> CELDRDPEGKDFQQPYTSFVQTKQNRDGLYALLRNTENPRMHFYQELQSDMYCTTITDGNSLAPFVNWDLGILNDHGRADEDEVSGIAGYYFVYNRLNQQANAFVNNTEAALQNQVYKNSTEIANAKSFLAEGKVLQALAIWRLMDRFSFHESVTEVNSGAKDLGVILLKEYNPGYIGPRATKAQCYDYILSRLSEAIEVLPENRESVLYVSRDYAYALRARIYLALGEYGKAAADAKMVVDKYPLIGAADASEFENIYRSDANNPEIIFRGFASATLGSFTATTLNGAAPAGKDIKYNPSAVPFQWVVDLYENEDFRKSVYIAKVVKKDKGYLVNKFLEDKAYRDVQDKPNLKVGARYFSVAEVYLILVESALQTGDTPTAEKYLKALSKARGAEVSVVNMEALQAERTRELIGEGSRLRDMVRWSIPNNHDAFETQPGLEGFANTTPLKAQAPVGFYAYTWEFPQRDRQTNPQLIKNWPI;> LSTVSGSVAKVSSEKLAEKPVANIMDALQGQVAGMQVMTTSGDPTAVASVEIHGTGSLGASSAPLYIVDGMQTSLDVVATMNPNDFESMSVLKDASATSIYGARAANGVVFIQTKKGKMSERGRITFNASYGISQILNTKPLDNMMTGDELLDFQVKAGFWGNNQTVQKVKDMILAGAEDLYGNYDSLKDEYGKTLFPVDFNHDADWLKALFKTAPTSQGDISFSGGSQGTSYYASIGYFDQEGMAREPANFKRYSGRLNFESRINEWLKVGANLSGAIANRRSADYFGKYYMGSGTFGVLTMPRYYNPFDVNGDLADVYYMYGATRPSMTEPYFAKMRPFSSESHQANVNGFAQITPIKGLTLKAQAGVDITNTRTSSKRMPNNPYDSTPLGERRERAYRDVSKSFTNTAEYKFSIDEKHDLTALMGHEYIEYEGDVIGASSKGFESDKLMLLSQGKTGNSLSLPEHRVAEYAYLSFFSRFNYGFDKWMYIDFSVRNDQSSRFGSNNRSAWFYSVGGMFDIYNKFIQESNWLSDLRLKMSYGTTGNSEIGNYNHQALVTVNNYTEDAMGLSISTAGNPD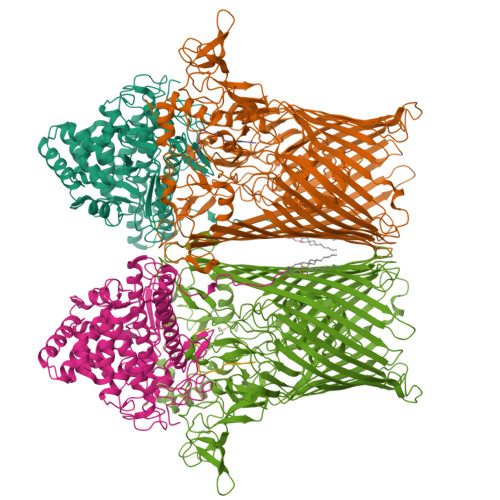LSWEKQSQFNFGLAAGAFNNRLSAEVDFYVRTTNDMLIDVPMPYISGFFSQYQNVGSMKNTGVDLSLKGTIYQNKDWNVYASANFNYNRQEITKLFFGLNKYMLPNTGTIWEIGYPNSFYMAEYAGIDKKTGKQLWYVPGQVDADGNKVTTSQYSADLETRIDKSVTPPITGGFSLGASWKGLSLDADFAYIVGKWMINNDRYFTENGGGLMQLNKDKMLLNAWTEDNKETDVPKLGQSPQFDTHLLENASFLRLKNLKLTYVLPNSLFAGQNVIGGARVYLMARNLLTVTKYKGFDPEAGGNVGKNQYPNSKQYVAGIQLSF;> GGATTATTTTSTS>MNIMRLLPRSKALSSPTAVAPAFRGRGAGVYSPSSQTVYMCPTSAVSLMHCSPCSTSAPLRSSQKSVAQTSANNDSLSDKFSAALAKNKEWAAKCSQEHPELLPTLAVGQHPEILWIGCSDSRCPETTILGLLPGDVFTHRNIANVIHPADLSSGAVIEFAVRHLRVKHVVICGH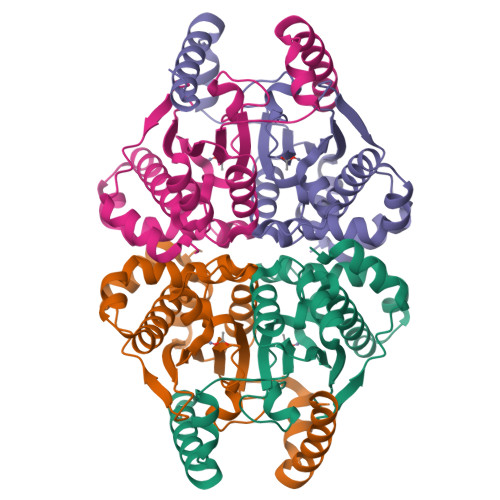TKCGGVAAALGNKGLGILDPWLIPLRQLREQHLAELQSLSRDEAVVRLAELNVKEGLKALTQKSVVLEAMQERGLQVHGLIYDVGSGFLRQLDAAEPEEALKARLTSFKTDA[4x]>MGRFVVWPSELDSRLSRKYGRIVPRSIAVESPRVEEIVRAAEELKFKVIRVEEDKLNPRLSGIDEELRTFGMIVLESPYGKSKSLKLIAQKIREFRRRSAGTLVPR[4x]

In all living cells the signal recognition particle (SRP) recognizes nascent polypeptides destined for secretion or membrane insertion as they emerge from translating ribosomes. As SRP binds to signal sequences emerging from the ribosomes, the resulting complex composed of the SRP and the ribosome-nascent chain complex is then targeted towards the membrane through the GTP-dependent interaction with the membrane-associated SRP receptor (SR also named FtsY in bacteria). We describe the X-ray structures of SRP54 and SRP19 the two protein constituting the proteinaceous core of the SRP from the hyperthermophilic archaeon Pyrococcus furiosus. SRP54 and SRP19 constitute the conserved core in all archaeal and eukaryotic SRPs.

We solved two distinct crystal forms of Pfu-SRP19. Two molecules of SRP19 associate in a dimer with an extended β-sheet surface built around the anti-parallel association of their respective β2 strands. The tetramer is organized around two dimers facing each other through their respective β-sheets at an angle of 45°. Pfu-SRP19 is characterized by a more extended β-sheet due to longer β2 and β3 strands when compared with all other available SRP19 structures. The structure is also characterized by two loops (L1 and L2). The loop L1, the primary RNA-binding surface is rigid and well defined in density whereas the loop L2 is disordered and absent in our final models. Superposition of our free SRP19 structure on the RNA-bound SRP19 structures reveals that the difference between free SRP19 and the RNA-bound forms lies exclusively in the conformation of the L2 loop region. The disordered L2 region of the “free” protein has a well-defined conformation in the RNA bound structures. The structure of free Pfu-SRP19 reveals a compact entity and suggests that this subunit acts as a molecular scaffold and a chaperone involved in assembly of the functional ribonucleoprotein particle. Through an induced fit mechanism involving the rearrangement of its disordered L2 loop, SRP19 assists proper folding of the SRP RNA and therefore favors subsequent binding of SRP54.3-{2,4-dimethyl-5-[(Z)-(2-oxo-1,2-dihydro-3H-indol-3-ylidene)methyl]-1H-pyrrol-3-yl}propanoic acid | C18 H18 N2 O3 | 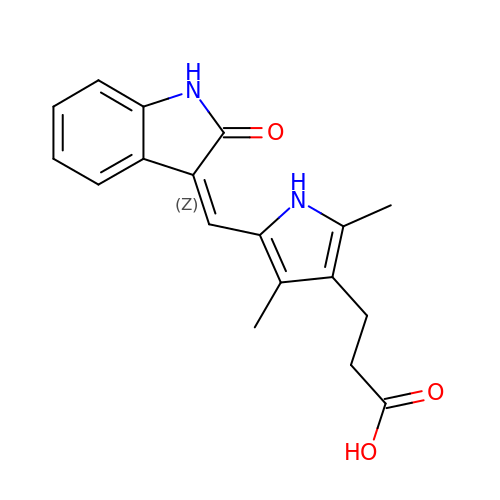NHFDRBXTEDBWCZ-ZROIWOOFSA-N>MTRTEIIRELERSLRLQLVLAIFLLALLIVLLWLLQQLKELLRELERLQREGSSDEDVRELLREIKELVENIVY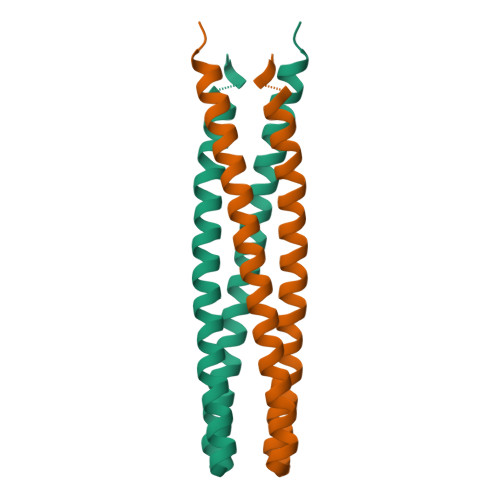LVIIIMVLVLVIIALAVTQKYLVEELKRQDLEHHHHH[4x]> G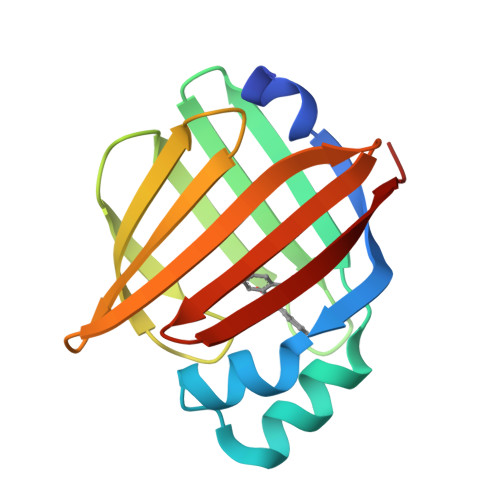SHMATVQQLEGRWRLVDSKGFDEYMKELGVGIALRKMGAMAKPDCIITCDGKNLTIKTESTLKTTQFSCTLGEKFEETTADGRKTQTVCNFTDGALVQHQEWDGKESTITRKLKDGKLVVECVMNNVTCTRIYEKVE>ATKVKYPDGFRSWYHVKSMVIQPGHPLENPFGGIHHVYANAEAIQGLRGGNYPDGAVLVFDLFDYQEDNHALVEGKRKLIGVMERDAKRFSATGGWGYEGFGEGKPDKRLVTDGGQGCFGCHAAQKESQYVFSRLRD[2x]

A widely applicable approach is the use of photocaged substrates, where the photocage is soaked into the crystal in advance and then activated using a laser pulse to provide uniform initiation of the reaction throughout the crystal. This work characterizes photocage release of nitric oxide and binding of this ligand to two heme protein systems, cytochrome c′-β and dye-decolourizing peroxidase B using a fixed target sample delivery system. In this work, we describe a thorough characterization of the application of the NO photocage N,N′-bis-(carb­oxy­methyl)-N,N′-di­nitroso-1,4-phenyl­enedi­amine (henceforth referred to as NO cage) to room-temperature microcrystals of two proteins: a gas binding cytochrome c′ (McCP-β) and a dye-decolourizing peroxidase B (DtpB). Laser parameters for photoactivation are systematically explored, and time-resolved structures over timescales ranging from 100 µs to 1.4 s using synchrotron and XFEL beamlines are described. We have demonstrated a sample and time efficient approach using fixed targets to carry out time-resolved SSX and SFX experiments with an NO photocage over the microsecond to second time regimes.

The first laser-initiated data collections used a delay time (1.44 s) much longer than the predicted NO release (microseconds; Section 2.1) and binding times [<1 ms;], for simple verification of NO release from our cage and successful binding to form a stable end-state complex. To establish suitable parameters for effective release of the photocage without the use of excessive laser power that could cause sample heating or multi-photon excitation effects, we conducted a laser power titration using the same fixed time delay of 1.44 s between laser and X-rays. Three SSX datasets were collected at different laser powers under otherwise identical conditions, at 9.5, 0.95 and 0.19 µJ (approximately 5, 0.5, 0.1 nJ µm−2), to resolutions of 2.00, 1.80 and 1.75 Å, respectively. These datasets yield similar protein structures, with full NO occupancy displayed in all of them, as shown in Fig. 5(c)–5(f). The binding of NO in the different structures exhibits a similar Fe—N bond length, and some variation in the Fe—N—O bond angle, but the direction in which the bent NO is oriented is not correlated with laser power. Instead, this is relatively poorly determined due to the difficulty of fitting the small diatomic ligand into the electron density. In McCP-β, we were able to show that the photocage successfully generated the initial distal six-coordinate species that is an end state in this protein but a transient intermediate in other cytochromes c′.> MADNMTTTQIEVGPGATNATINFEAGILECYERFSWQRALDYPGQDRLHRLKR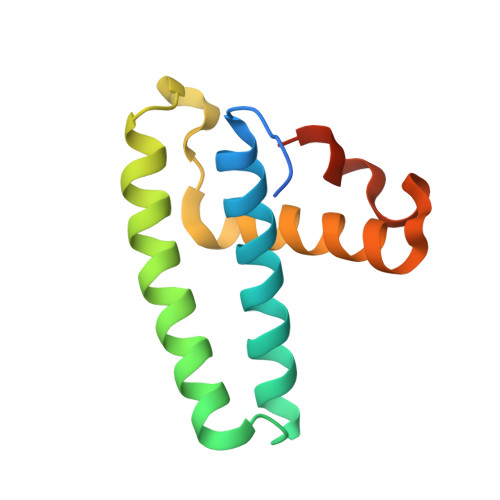KLESRIKTHNKSEPENKRMSLEERKAIGVKMMKVLLFMDPSAGIEGFEPYHHHHHH>MSGIIATYLIHDDSHNLEKKAEQIALGLTIGSWTHLPHLLQEQLKQHKGNVIHVEELAEHEHTNSYLRKKVKRGIIKIEYPLLNFSPDLPAILTTTFGKLSLDGEVKLIDLTFSDELKKHFPGPKFGIDGIRNLLQVHDRPLLMSIFKGMIGRNIGYLKTQLRDQAIGGVDIVKDDEILFE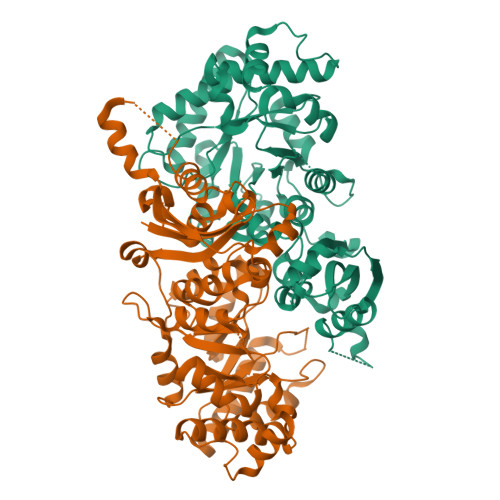NALTPLTKRIVSGKEVLQSVYETYGHKTLYAVNLTGRTFDLKENAKRAVQAGADILLFNVFAYGLDVLQSLAEDDEIPVPIMAHPAVSGAYSASKLYGVSSPLLLGKLLRYAGADFSLFPSPYGSVALEKEEALAISKYLTEDDASFKKSFSVPSAGIHPGFVPFIVRDFGKDVVINAGGGIHGHPNGAQGGGKAFRTAIDATLQNKPLHEVDDINLHSALQIWGNPSYEVKL[2x]>MHHHHHHKNIINTSILNLRYESNHLIDLSRYASEINIGSKVNFDPIDKNQIQLFNLESSKIEIILKNAIVYNSMYENFSTSFWIKIPKYFSKINLNNEYTIINCIENNSGWKVSLNYGEIIWTLQDNKQNIQRVVFKYSQMVAISDYINRWIFITITNNRLNNSKIYINGRLIDQKPISNLGNIHASNNIMFKLDGCRDPHRYIWIKYFNLFDKELNEKEIKDLYDNQSNSGILKDFWGNYLQYDKPYYMLNLYDPNKYVDVNNVGIRGYMYLKGPRGSIVTTNIYLNSSLYMGTKFIIKKYASGNKDNIVRNNDRVYINVVVKNKEYRLATNASQAGVEKILSVLEIPDVGNLSQVVVMKSKNDQGIRNKCKMNLQDNNGNDIGFIGFHQFNNIDKLVASNWYNRQIERSSRTFGCSWEFIPVDDGWGESPL[2x]

Botulinum neurotoxins (BoNT) cause the potentially fatal neuroparalytic disease botulism that arises due to proteolysis of a SNARE protein. Each BoNT is comprised of three domains: a cell binding domain (HC), a translocation domain (HN), and a catalytic (Zn2+ endopeptidase) domain (LC). The HC is responsible for neuronal specificity by targeting both a protein and ganglioside receptor at the neuromuscular junction. Here we present the crystal structures of two BoNT cell binding domains, HC/A4 and HC/A5, in a complex with the oligosaccharide of ganglioside, GD1a and GM1b, respectively.

Several attempts to crystallise HC/A5 with GD1a did not yield crystals for the complex. Consequently, a smaller ganglioside, GM1b, which is identical to GD1a in terms of the expected binding portion (Sia5-GalNAc3) but lacks only Sia6, was used for co-crystallisation with HC/A5. Crystals of HC/A5:GM1b diffracted to 2.4 Å, in space group P21, and the structure was determined by molecular replacement with two molecules (designated A and B) in the ASU. For molecule A, some additional weak electron density was observed at the GBS that was not part of the protein. With the aid of polder maps for His 1253 and Tyr 1117, it was possible to model in sugars Gal4 and Sia5. Gal4 forms a total of four hydrogen bonds with residues Glu 1203, Phe 1252, His 1253, and Ser 1264, while Sia5 forms three hydrogen bonds with Tyr 1117, Tyr 1267, and Gly 1279. Further refinement of the Gal4 molecule with occupancies 0.6 and 1 generated average B-factors of 60.74 Å2 and 61.97 Å2, respectively, indicating that GM1b is bound at low occupancy. Considering that the residues of the GBS for molecule B could not be modelled, comparisons to the unbound HC/A5 structure will be made with molecule A. Most of the residues within the putative GBS show little to no conformational change, with the exception of Phe 1278 which has its side chain flipped towards the GBS. This flip in residue positioning is accompanied by a change in the loop structure spanning residues 1260-1280, where there is an increase in the Cα distance of 4 Å between residues Tyr 1267 and Thr 1277 upon ganglioside binding (B inset). The low occupancy of GM1b, and multiple failed attempts of co-crystallising HC/A5 with GD1a, suggested a low affinity to the Sia-Gal-GalNAc moiety or preference for a different ganglioside.> GGA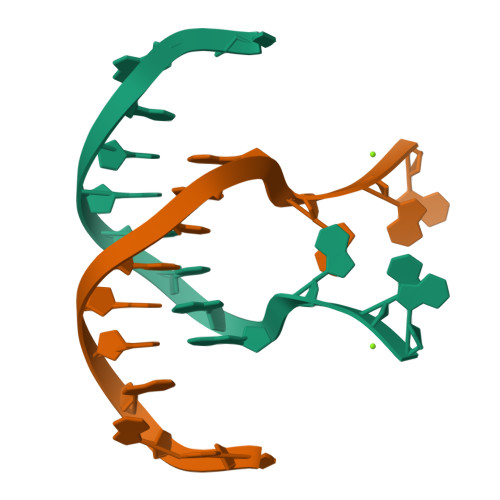AACGTTGGAG> GPGMRVSGSASSQDIISRINSKNINNNDSNEVKRIKDALSIESKERILYPQNLSRDNLKQMARYVNNTYVHYSGNCVLLSACLHYNIHHRQDILSSKNTASPTVGL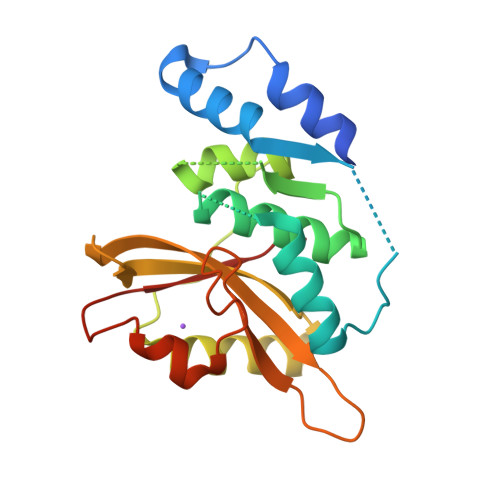DSAIVDKIIFGHELNQSYSLNSIDEVEKEILNRYDIKRESSFIISAENYIAPIIGESRHDFNAVVISEYDKKPYVQFIDSWKTSNILPSLQEIKKHFSSSGEFYVRAYDEKHD> IPVIEPLFTKVTEDIPGAEGPVFDKNGDFYIVAPEVEVNGKPAGEILRIDLKTGKKTVICKPEVNGYGGIPAGCQCDRDA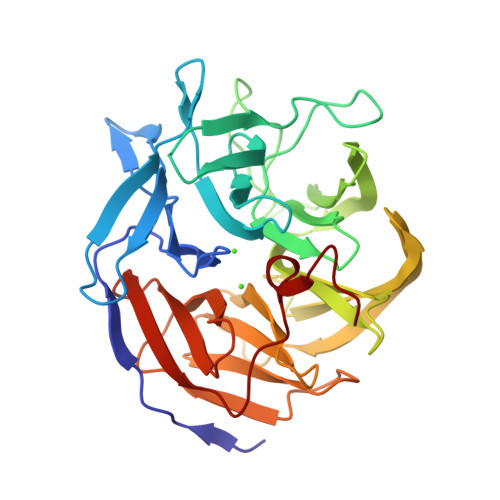NQLFVADMRLGLLVVQTDGTFEEIAKKDSEGRRMQGCNDCAFDYEGNLWITAPAGEVAPADYTRSMQEKFGSIYCFTTDGQMIQVDTAFQFPNGIAVRHMNDGRPYQLIVAETPTKKLWSYDIKGPAKIENKKVWGHIPGTHEGGADGMDFDEDNNLLVANWGSSHIEVFGPDGGQPKMRIRCPFEKPANLHFKPQTKTIFVTEHENNAVWKFEWQRNGKKQYCETLKFGIF>MKIALINENSQASKNTIIYKELKAVSDEKGFEVFNYGMYGKEEESQLTYVQNGLLTAILLNSGAADFVITGCGAGIGAMLACNSFPGVVCGFAADPVDAYLFSQVNGGNALSLPFAKGFGWGAELNLRYLFERLFEDEKGGGYPKERAVPEQRNARILSEIKQITYRDL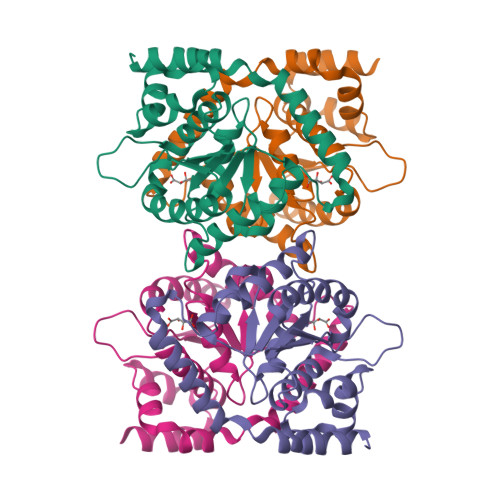LSVLKEIDQDFLKETISGEHFQEYFFANCQNQNIADYLKSVLDLEHHHHHH[2x]3-(furan-2-yl)propanoic acid 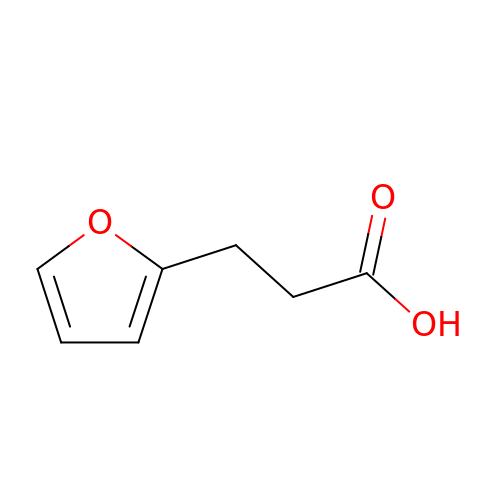| C7 H8 O3 | XLTJXJJMUFDQEZ-UHFFFAOYSA-N> GTTGGGGTTGGGGTTGGG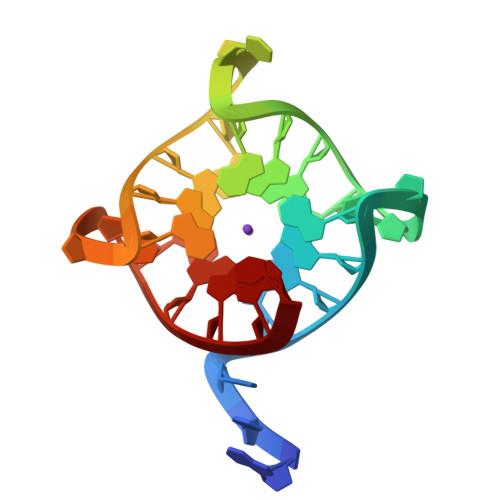GTTGGGGT>MRSDTSVEPEGANFIAEFFGHRVYPEVVSTEAARNDQATGTCPFLTAAKLVETSCVKAETSRGVCVVNTAVDNERYDWLVCPNRALDPLFMSAASRKLFGYGPTEPLQFIAAPTLADQAVRDGIREWLDRGVHVVAYFQEKLGGELSISKTDSSPEFSFDWTLAEVESIYPVPKIKRYGVLEIQTMDFHGSYKHAVGAIDIALVEGIDFHGWLPTPAGRAALSKKMEGPNLSNVFKRTFYQMAYKFALSGHQRCAGTGFAIPQSVWKSWLRHLANPTLIDNGDGTFSLGDTRNDSENAWIFVFELDPDTDASPRPLAPHLEIRVNVDTLIDLALRESPRAALGPSGPVATFTDKVE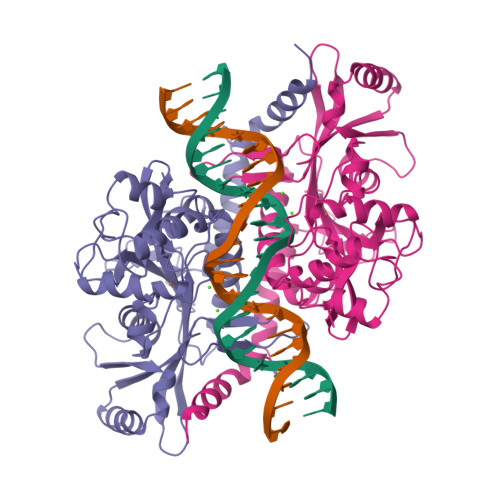ARMLRFWPKTRRRRSTTPGGQRGLFDA[2x]> SNAMSLILDDIILSLTNANERTPPQALKTTLSLLYEKSKQYGLSSPQLQALVRLLCETSIIDTVTKVYIVENCFLPDGYLTKELLLEIINHLGTPTVFSRYRIQTPPVLQSALCKWLVHVYFLFPVHSEREHNISSSIWLHLWQFSFLQKWITPLVIWQATTPVDVKPWKLSIIKRCAMHPGYRDAPGSATLILQRFQCLVGASSQITESIITINCNRKTLKSHRNLKLDAHFLSILKRILSRAHPANFPADTVQNTIDMYLSEIHQLGADSIYPLRLQSLPEYVPSDSTVSLWDVTSLEQLAQNWPQLHIPNDVDYMMKPSLNSNVLLPRKVMSRDSLKHLYSSIILIKNSRDESSSPYEWCIWQLKRCFAHQIETPQEVIPIIISVS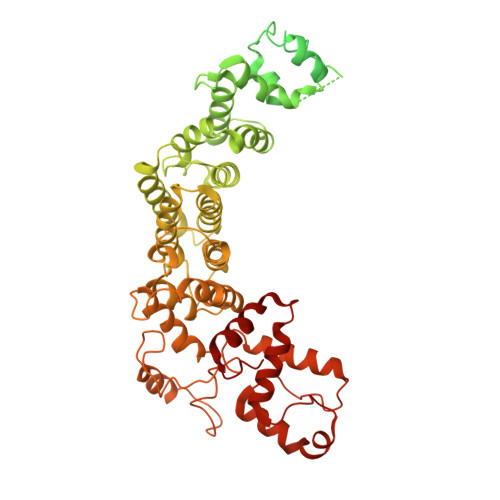SMDNKLSSRIIQTFCNLKYLKLDELTLKKVCGGILPLWKPELISGTREFFVKFMASIFMWSTRDGHDNNCTFSETCFYVLQMITNWVLDDKLIALGLTLLHDMQSLLTLDKIFNNATSNRFSTMAFISSLDILTQLSKQTKSDYAIQYLIVGPDIMNKVFSSDDPLLLSAACRYLVATKNKLMQYPSTNKFVRMQNQYIMDLTNYLYRNKVLSSKSLFGVSPDFFKQILENLYIPTADFKNAKFFTITGIPALSYICIIILRRLETAENTKIKFTSGIINEETFNNFFRVHHDEIGQHGWIKGVNNIHDLRVKILMHLSNTANPYRDIAAFLFTYLKSLSKYSVQNS>ASTKAQPTEVSSILEERIKGVSDEANLNETGRVLAVGDGIARVFGLNNIQAEELVEFSSGVKGMALNLEPGQVGIVLFGSDRLVKEGELVKRTGNIVDVPVGPGLLGRVVDALGNPIDGKGPIDAAGRSRAQVKAPGILPRRSVHEPVQTGLKAVDALVPIGRGQRELIIGDRQTGKTAVALDTILNQKRWNNGSDESKKLYCVYVAVGQKRSTVAQLVQTLEQHDAMKYSIIVAATASEAAPLQYLAPFTAASIGEWFRDNGKHALIVYDDLSKQAVAYRQLSLLLRRPPGREAYPGDVFYLHSRLLERAAKLSEKEGSGSLTALPVIETQGGDVSAYIPTNVISITDGQIFLEAELFYKGIRPAINVGLSVSRVGSAAQVKALKQVAGSLKLFLAQYREVAAFAQFGSDLDASTKQTLVRGERLTQLLKQNQYSPLATEEQVPLIYAGVNGHLDGIELSRIGEFESSFLSYLKSNHNELLTEIREKGELSKELLASLKSATESFVATF[6x];>[6x]ASAAQSTPITGKVTAVIGAIVDVHFEQSELPAILNALEIKTPQGKLVLEVAQHLGENTVRTIAMDGTEGLVRGEKVLDTGGPISVPVGRETLGRIINVIGEPIDERGPIKSKLRKPIHADPPSFAEQSTSAEILETGIKVVDLLAPYARGGKIGLFGGAGVGKTVFIQELINNIAKAHGGFSVFTGVGERTREGNDLYREMKETGVINLEGESKVALVFGQMNEPPGARARVALTGLTIAEYFRDEEGQDVLLFIDNIFRFTQAGSEVSALLGRIPSAVGYQPTLATDMGLLQERITTTKKGSVTSVQAVYVPADDLTDPAPATTFAHLDATTVLSRGISELGIYPAVDPLDSKSRLLDAAVVGQEHYDVASKVQETLQTYKSLQDIIAILGMDELSEQDKLTVERARKIQRFLSQPFAVAEVFTGIPGKLVRLKDTVASFKAVLEGKYDNIPEHAFYMVGGIEDVVAKAEKLAAEAN;>ATLKEVEMRLKSIKNIEKITKTMKIVASTRLSKAEKAKISAKKMDEAEQLFYKNAETKNLDVEATETGAPKELIVAITSDKGLCGSIHSQLAKAVRRHLNDQPNADIVTIGDKIKMQLLRTHPNNIKLSINGIGKDAPTFQESALIADKLLSVMKAGTYPKISIFYNDPVSSLSFEPSEKPIFNAKTIEQSPSFGKFEIDTDANVPRDLFEYTLANQMLTAMAQGYAAEISARRNAMDNASKNAGDMINRYSILYNRTRQAVITNELVDIITGASSLG[2x];>AEAAAASSGLKLQFALPHETLYSGSEVTQVNLPAKSGRIGVLANHVPTVEQLLPGVVEVMEGSNSKKFFISGGFATVQPDSQLCVTAIEAFPLESFSQENIKNLLAEAKKNVSSSDAREAAEAAIQVEVLENLQSVLK[2x];>SAWRKAGISYAAYLNVAAQAIRSSLKTELQTASVLNRSQTDAFYTQYKNGTAASEPTPITK[2x];>SEGSTGTPRGSGSEDSFVKRARATEDFFVRQREKEQLRHLKEQLEKQRKKIDSLENKIDSMTK[2x]

The hydrolysis of ATP by the F-ATPase isolated from mitochondria is inhibited by a small basic protein, known as IF1. The binding of IF1 to the enzyme requires the hydrolysis of ATP to drive the anticlockwise rotation of the central stalk (as viewed from the membrane domain of the intact enzyme) and entrap the inhibitor in its binding site. The ATPase inhibitor protein from Saccharomyces cerevisiae is 63 amino acids long. The poorly conserved N-terminal region (residues 1–16), is followed by a well-conserved segment from residues 17 to 45, corresponding to the long α-helix in the inhibitory region of the bovine protein.

The models of both assemblies in the asymmetric unit contain the same residues and have the same nucleotide occupancy. Residues 17–35 of the α-helix are bound into a deep groove between the C-terminal domains of the αDP- and βDP-subunits. Residues 1–5 of the inhibitor are in the aqueous chamber surrounding the γ-subunit in the central region of the F1-domain. Residues 6–16 form a loop region held together by a salt bridge between residues R9 and D15 of the inhibitor, and by a hydrogen-bonding network involving residues S4, R9 and D15 of the inhibitor. However, the other interactions noted in the bovine complex are not conserved, but the structure indicates that there are additional significant interactions that are specific to the yeast complex. They are a salt bridge between residue E2 of the inhibitor with residue K361 in α-helix H of the αE-subunit, and between R32 of the inhibitor and E398 and E405 in the βDP-subunit, and an electrostatic interaction between inhibitor residue D15 and R9 in the γ-subunit. In the bovine structure, there is no nucleotide bound to this subunit, whereas in the yeast complex, the still partially formed nucleotide binding site of the βE-subunit is occupied by ADP, but without an accompanying bound magnesium ion, despite the presence of 13 mM magnesium sulphate during formation and crystallization of the inhibited complex. However, the amino acid side chains that are involved in coordinating a magnesium ion indirectly by binding ligand water molecules (βE189, βE193 and βD256) have moved away from the positions that provide the coordinating environment (as found in the βDP- and βTP-subunits), and the magnesium ion has been released from the βE-subunit. Thus, the present structure indicates that the magnesium ion is released before ADP, and that the inhibitor has arrested the catalytic cycle of ATP hydrolysis immediately preceding the release of the nucleotide.> MGHHHHHHMQVADKHELGQLQYSLDYDFQSGQLLVGILQAMGLAALDLGGSSDPYVRVYLLPDKRRR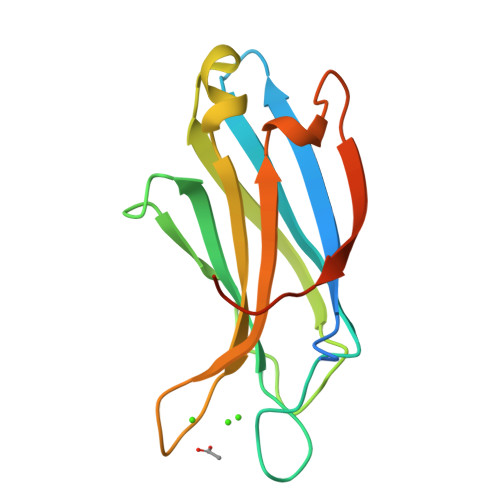YETKVHRQTLNPHFGETFAFKVPYVELGGRVLVMAVYDFDRFSRNDAIGEVRVPMSSVDLGRPVQAWRELQAAPREEQEKLGD>[4x]GSHMNLFVA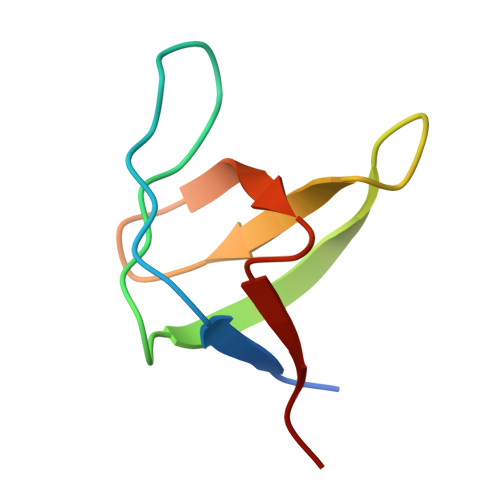LYDFVASGDNTLSITKGEKLRVLGYNQNGEWSEVRSKNGQGWVPSNYITPVN> GPMPGKSVVARVAEAYPEDVGKRIVR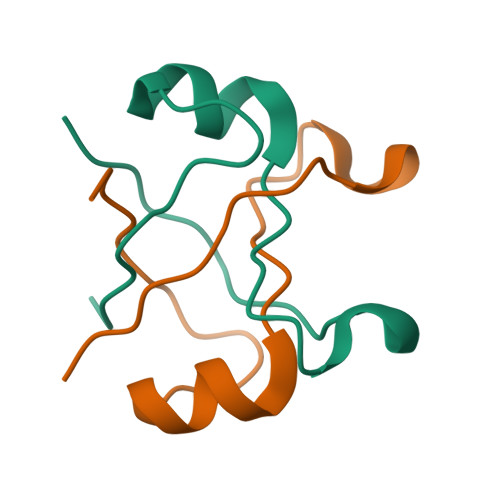MDKYERAKLGVSVGDYVEVKKV Protein-engineering methods have been exploited to produce a surrogate system for the extracellular neurotransmitter-binding site of a heteromeric human ligand-gated ion channel, the glycine receptor. Acetylcholine-binding protein is a highly conserved ortholog of the pLGIC extracellular ligand-binding domain (ECD) with properties similar to nAChR. Mutations affecting key residues in the orthosteric agonist site at the α1(−)/β(+) interface affect the potency of both activation by glycine and inhibition by strychnine. We therefore set out to generate a high-fidelity surrogate of this α1(−)/β(+) orthosteric binding site using the 2α1:3β stoich­iometry [Fig. 1(a)] by exploiting protein-engineering methods and the thermal stability of acetylcholine-binding protein from Aplysia californica (AcAChBP). Ultimately, the highly stable AcAChBP framework has allowed us to introduce nine amino-acid substitutions that have resulted in a stable surrogate for a heteromeric neurotransmitter site that binds glycine.

The structure of the GBP–strychnine complex displays a well ordered ligand in three out of five binding sites per asymmetric unit. In two sites the density is less clear, the thermal parameters are elevated and different strychnine orientations are noted. An overlay of the protein structures (data not shown) places the tertiary amines within 2 Å of each other, but the ligands adopt different poses, essentially pivoting around this N atom. In the GBP–strychnine complex the tertiary amine is protonated and donates a hydrogen bond to a highly ordered water that forms hydrogen bonds to the carbonyl groups of Ser163 and Tyr166 and contributes to a solvent network that burrows into the protein fold (data not shown). The G162E change directs a polar side chain into the bindng site and this forces the strychnine to adopt a different orientation. The change in orientation of strychnine results in the amide carbonyl O atom rotating by about 90° and relocating by almost 8 Å directed towards Met133 and with the indole system placed to interact with loop C. Here also there are significant changes to the protein structure. The side chain of Tyr205 adopts a different rotamer, participates in van der Waals interactions with strychnine and now occupies the space that is filled by the Cys207–Cys208 disulfide bond in WT AcAChBP, in essence forming a lid over the binding site. Tyr212 also displays a different rotamer, partially filling the space vacated by Tyr205, and this allows the strychnine indole moiety to bind under loop C. The substitutions that were introduced to engineer a glycine-binding site in GBP have however reduced the affinity for strychnine significantly away from that of the wild-type template as well as from that observed with recombinant homomeric GlyR samples.

>[5x]MLVSVYLALLVACVGQAHSQANLMRLKSDLFNRSPMYPGPTKDDPLTVTLGFFLQDIVKVDSSTNEVDLVYYERQRWKLNSLMWDPNEYGNITDFRTSAADIWTPDITAASSTRPVQVLSPQIAVVTHDGSVMFSPAQRLSFMCDPTGVDSEEGVTCAVKFESWVYSGFEIDLKTDTDQVDLSSYYASSKYEILSATQTRQVQHYKGTGEPYIDVNLVVKFRERRAGNGFFRNLFDENLYFQGHHHHHH The completed linker tetrasaccharide represents the point of bifurcation in GAG biosynthesis: either EXTL3 adds an α-linked GlcNAc and initiates HS polymerisation or one of two closely related CSGALNACTs adds a β-linked GalNAc and initiates CS polymerisation. We show that selection of the GAG chain type occurs at the priming step: CSGALNACTs are capable of initiating CS synthesis on all GAG attachment sites, whereas EXTL3 requires specific features in the core protein to initiate HS synthesis. Structure-function analysis reveals that acidic residues in the glycopeptide substrate and a basic exosite in EXTL3 are critical for specifying HS biosynthesis. Our results demonstrate that modification with CS occurs by default and must be overridden by EXTL3 to produce HS.

In order to explain these data mechanistically, we determined crystal structures of an EXTL3 dimer lacking the coiled-coil (residues 154–919) in the apo form (1.58 Å resolution) and with UDP and Mn2+ bound (2.10 Å resolution). The latter structure was obtained by crystal soaking that also included TetraP-BETA, but unfortunately the glycopeptide was excluded from the GlcNAc transferase site by a crystal lattice contact. The large dimer interface features an intermolecular disulfide bond (Cys793–Cys915) that staples the C-terminal tail of one subunit to the body of the other subunit. In this model, only the terminal GlcA is enclosed by the enzyme; all other linker sugars are surprisingly exposed (even the GlcA is less buried than in EXTL2 due to a Trp-to-Ser substitution in EXTL3). The Xyl2P phosphate group is ≈20 Å away from the GlcNAc transferase site and close to Arg907. This arginine is part of a large basic surface region spanning the dimer interface that has been suggested to interact with the peptide portion of acceptor substrates. We found that EXTL3 specificity is determined by a basic exosite >20 Å from the GlcNAc transferase site. The failure of EXTL3 to polymerise a long HS backbone is likely to be the result of weak acceptor binding at the GlcNAc transferase site: without assistance from the exosite, longer acceptor glycans are likely to have very high KM values, preventing efficient elongation.

>[2x]APLVHHHHHHALDENLYFQGALATTLDEADEAGKRIFGPRVGNELCEVKHVLDLCRIRESVSEELLQLEAKRQELNSEIAKLNLKIEACKKSIENAKQDLLQLKNVISQTEHSYKELMAQNQPKLSLPIRLLPEKDDAGLPPPKATRGCRLHNCFDYSRCPLTSGFPVYVYDSDQFVFGSYLDPLVKQAFQATARANVYVTENADIACLYVILVGEMQEPVVLRPAELEKQLYSLPHWRTDGHNHVIINLSRKSDTQNLLYNVSTGRAMVAQSTFYTVQYRPGFDLVVSPLVHAMSEPNFMEIPPQVPVKRKYLFTFQGEKIESLRSSLQEARSFEEEMEGDPPADYDDRIIATLKAVQDSKLDQVLVEFTCKNQPKPSLPTEWALCGEREDRLELLKLSTFALIITPGDPRLVISSGCATRLFEALEVGAVPVVLGEQVQLPYQDMLQWNEAALVVPKPRVTEVHFLLRSLSDSDLLAMRRQGRFLWETYFSTADSIFNTVLAMIRTRIQIPAAPIREEAAAEIPHRSGKAAGTDPNMADNGDLDLGPVETEPPYASPRYLRNFTLTVTDFYRSWNCAPGPFHLFPHTPFDPVLPSEAKFLGSGTGFRPIGGGAGGSGKEFQAALGGNVPREQFTVVMLTYEREEVLMNSLERLNGLPYLNKVVVVWNSPKLPSEDLLWPDIGVPIMVVRTEKNSLNNRFLPWNEIETEAILSIDDDAHLRHDEIMFGFRVWREARDRIVGFPGRYHAWDIPHQSWLYNSNYSCELSMVLTGAAFFHKYYAYLYSYVMPQAIRDMVDEYINCEDIAMNFLVSHITRKPPIKVTSRWTFRCPGCPQALSHDDSHFHERHKCINFFVKVYGYMPLLYTQFRVDSVLFKTRLPHDKTKCFKFI(5R)-5-[(7-chloro-1H-indol-3-yl)methyl]-3-methylimidazolidine-2,4-dione 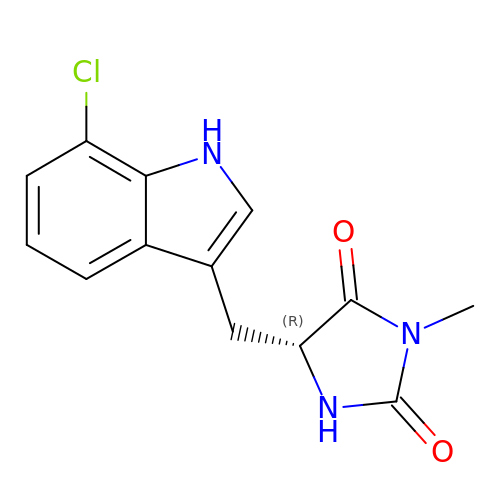| C13 H12 Cl N3 O2 | WIKGAEMMNQTUGL-SNVBAGLBSA-N> MASVIKPTQYKPVPDEEPNSTDVEETLERIKNNDPKLEEVNLNNIRNIPIPTLKAYAEALKENSYVKKFALANTRADDHVAFAIAIMLKANKTITSLNLDSNHITGKGILAIFRALLQNNTLTELRFHNQ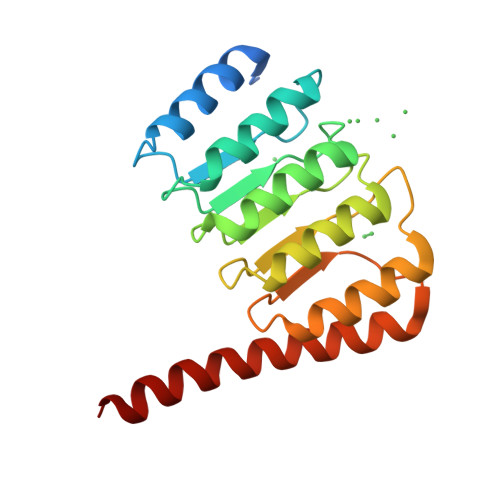RHICGGKTEMEIAKLLKENTTLLKLGYHFELAGPRMTVTNLLSRNMDKQRQKRLQEQRQAQ N-methyl-4-[4-({[3-(trifluoromethyl)phenyl]carbamoyl}amino)phenoxy]pyridine-2-carboxamide | C21 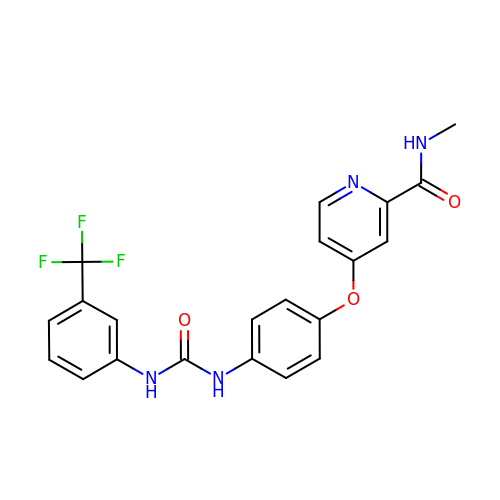H17 F3 N4 O3 | WFTZMAAMCVPJJT-UHFFFAOYSA-N The growth/motility factor hepatocyte growth factor/scatter factor (HGF/SF) and its receptor, the tyrosine kinase MET, constitute a signalling system essential for embryogenesis and for tissue/organ regeneration in post-natal life. Two truncated forms of HGF/SF are produced by alternative splicing of the primary transcript: NK1 encodes the N domain and the first K domain (K1),16 while NK2 encodes the N, K1 and K2 domains. NK1 is a monomer in solution, but crystallises as a head-to-tail dimer and all available crystal structures of human and mouse NK1 yielded the same dimer. (c) The lysine-binding pocket of the kringle domain of NK1 is formed by a glycine loop at the top of pocket (E183 and G186), an aromatic “base” (W188) and sides (F162 and Y198), as well as a positively charged anchor at the bottom of the pocket (R197).

In initial experiments HEPES was successfully incorporated into apo NK1 crystals by soaking and bound into the lysine-binding pocket in a mode consistent with previous results. The piperazine moiety of HEPES makes strong carbon and donor π-interactions with W188 and Y198, and weak polar interactions with E183, whereas the hydroxyl group engages the glycine loop in weak polar interactions. A HEPES molecule is bound in the pocket and shown with its carbon atoms in dark gray and its sulphur atom in yellow. Hydrogen bonds between the HEPES molecule and NK1 are represented by dashed lines. All of the compounds discussed here, as confirmed by crystallographic analysis, show the conserved and crucial hydrogen bonds to R197 and the differences in binding affinity reflect additional interactions. This is demonstrated, for example, by HEPES (KD = 2.4 mM) which, compared to (H)EPPS (KD = 7.0 mM) and PIPES (KD = 26.6 mM), forms stronger π-interactions to W188 an Y198, weak polar interactions to E183 and further contacts with the glycine loop. Binding constants obtained from SPR and NMR are comparable and the figures indicate that CAPS and HEPES display the highest binding affinities, whereas PIPES and CHES display the lowest. Inhibition of phosphorylation of Erk 1/2 and Akt (S473) was seen for HEPES, (H)EPPS, MES, MOPS and CAPS at the highest concentration (100 mM, lanes 4).

>YVEGQRKRRNTIHEFKKSAKTTLIKIDPALKIKTKKVNTADQCANRCTRNKGLPFTCKAFVFDKARKQCLWFPFNSMSSGVKKEFGHEFDLYENKDYIRNCIIGKGRSYKGTVSITKSGIKCQPWSSMIPHEHSFLPSSYRGKDLQENYCRNPRGEEGGPWCFTSNPEVRYEVCDIPQCSEVE[2x]>HYTWPRVNDGADWQQVRKADNWQDNGYVGDVTSPQIRCFQATPSPAPSVLNTTAGSTVTYWANPDVYHPGPVQFYMARVPDGEDINSWNGDGAVWFKVYEDHPTFGAQLTWPSTGKSSFAVPIPPCIKSGYYLLRAEQIGLHVAQS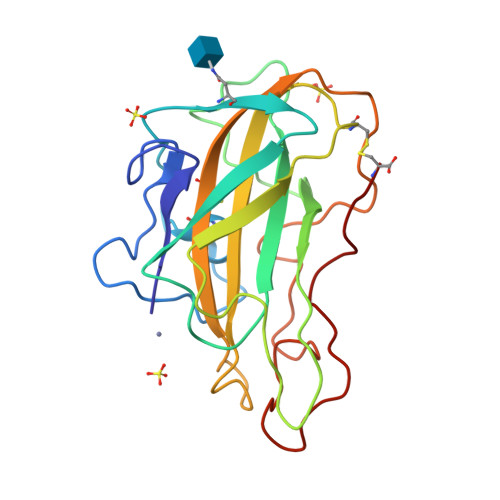VGGAQFYISCAQLSVTGGGSTEPPNKVAFPGAYSATDPGILINIYYPVPTSYQNPGPAVFSC[4x]>SFVEMVDNLRGKSGQGYYVEMTVGSPPQTLNILVDTGSSNFAVGAAPHPFLHRYYQRQLSSTYRDLRKGVYVPYTQGKWEGELGTDLVSIPHGPNVTVRANIAAITESDKFFINGSNWEGILGLAYAEIARPDDSLEPFFDSLVKQTHVPNLFSLQLCGAGFPLNQSEVLASVGGSMIIGGIDHSLYTGSLWYTPIRREWYYEV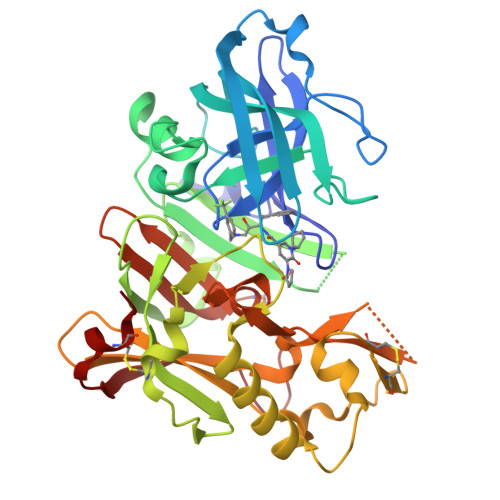IIVRVEINGQDLKMDCKEYNYDKSIVDSGTTNLRLPKKVFEAAVKSIKAASSTEKFPDGFWLGEQLVCWQAGTTPWNIFPVISLYLMGEVTNQSFRITILPQQYLRPVEDVATSQDDCYKFAISQSSTGTVMGAVIMEGFYVVFDRARKRIGFAVSACHVHDEFRTAAVEGPFVTLDMEDCGYN[3x]> GAMGGSEFPKSRLPTLADNEIEYEKQIGKGGFGLVHKGRLVKDKSVVAIKSLILGDSEGETEMIEKFQEFQREVFIMSNLNHPNIVKLYGLMHNPPRMVMEFVPCGDLYHRLLDKAHPIKWSVKLRLMLDIALGIEYMQNQNPPIVHRDLRSPNIFLQSLDENAPVCAKVADFGLSQQSVHSVSGLLGNFQWMAPETIGAEEESYTEKADTYSFAMILYTILTGEGPFDEYSYGKIKFINMIREEGLRPTIPEDCPPRLRNVIELCWSGDPKKRPHFSYIVKELS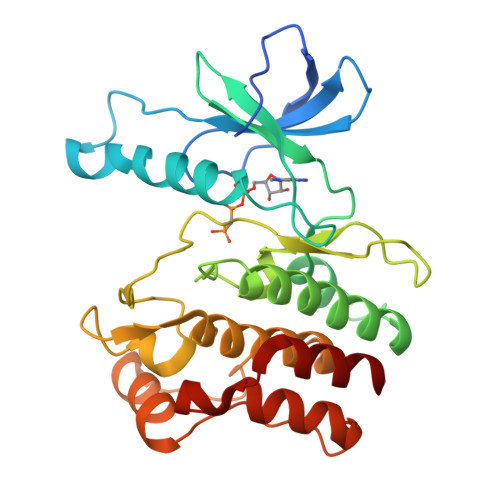EL> GDDNSYSLGDIWIAVATVVPEGNNVYYLRLDDGDKLWPAATNYPNYQPKPNQRALV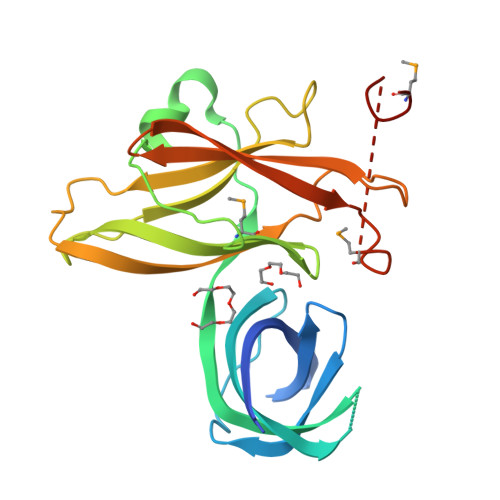NFTILADSTQSNLGGFSHYIKVNAIHNILTKSIAKNEGAANDSIYGTDPVSIYNNNMWIGDGYLNIYFETLWGGKTAHFINLIQPDAENDPYTLEFRHNAYDDPQYTIGAGRVAFNLSSLPDTKGETVDLVVNYWTSEGKQAYKLKYNSDKTKMEDTSQGYTNDSISNITDMK(2~{R})-2-[3,4-bis(oxidanyl)phenyl]-6-oxidanyl-2,3-dihydrochromen-4-one | C15 H12 O5 | 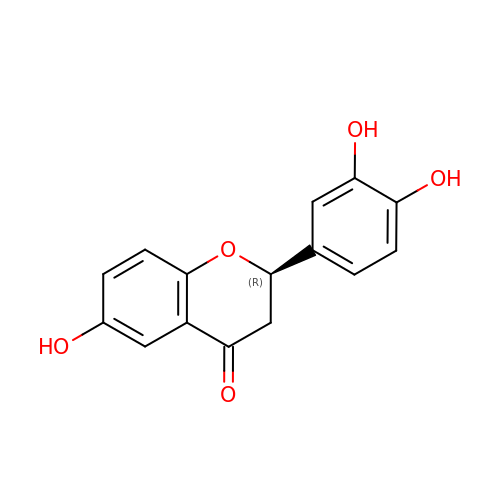SHYJMIHVPPCBNP-OAHLLOKOSA-N>GPHMTNPVVFFDVCADGEPLGRITMELFSNIVPRTAENFRALCTGEKGFGFKNSIFHRVIPDFVCQGGDITKHDGTGGQSIYGDKFEDENFDVKHTGPGLLSMANQGQNTNNSQFVITLKKAEHLDFKHVVFGFVKDGMDTV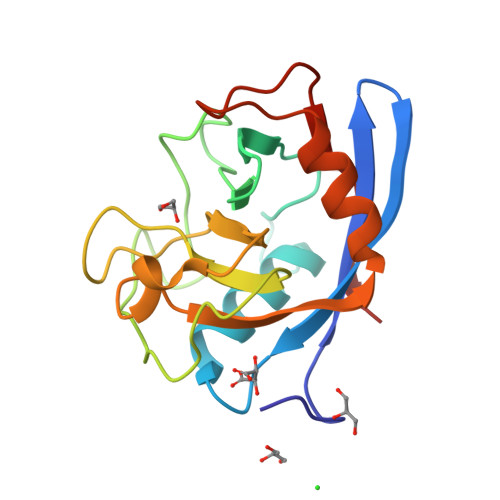KKIESFGSPKGSVCRRITITECGQI[6x]>MGSDKIHHHHHHMNVAILLAAGKGERMSENVPKQFLEIEGRMLFEYPLSTFLKSEAIDGVVIVTRREWFEVVEKRVFHEKVLGIVEGGDTRSQSVRSALEFLEKFSPSYVLVHDSARPFLRKKHVSEVLRRARETGAATLALKNSDALVRVENDRIEYIPRKGVYRILTPQAFSYEILKKAHENGGEWADDTEPVQKLGVKIALV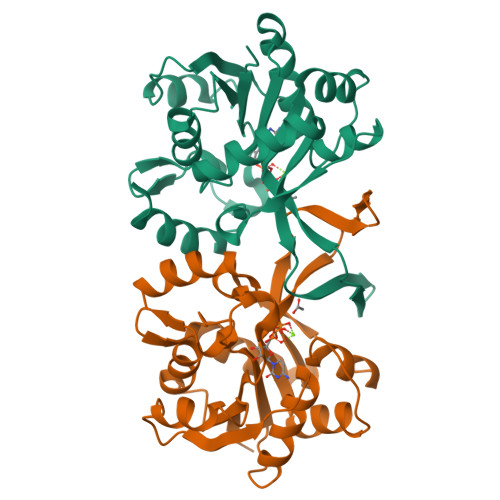EGDPLCFKVTFKEDLELARIIAREWERIP[2x]> MASMETSSSCESLGSQPAAARPPSVDSLSSASTSHSENSVHTKSASVVSSDSISTSADNFSPDLRVLRESNKLAEMEEPPLLPGENIKDMAKDVTYICPFTGAVRGTLTVTNYRLYFKSMERDPPFVLDASLGVINRVEKIGGASSRGENSYGLETVCKDIRNLRFAHKPEGRTRRSIFENLMKYAFPVSNNLPLFAFEYKEVFPENGWKLYDPLLEYRRQGIPNESWRITKINERYELCDTYPALLVVPANIPDEELKRVASFR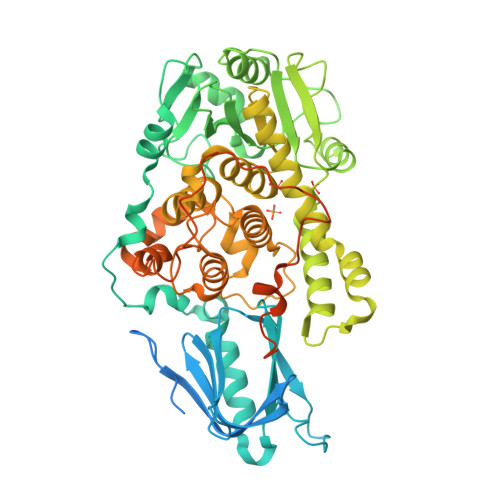SRGRIPVLSWIHPESQATITRCSQPMVGVSGKRSKEDEKYLQAIMDSNAQSHKIFIFDARPSVNAVANKAKGGGYESEDAYQNAELVFLDIHNIHVMRESLRKLKEIVYPNIEETHWLSNLESTHWLEHIKLILAGALRIADKVESGKTSVVVHSSDGWDRTAQLTSLAMLMLDGYYRTIRGFEVLVEKEWLSFGHRFQLRVGHGDKNHADADRSPVFLQFIDCVWQMTRQFPTAFEFNEYFLITILDHLYSCLFGTFLCNSEQQRGKENLPKRTVSLWSYINSQLEDFTNPLYGSYSNHVLYPVASMRHLELWVGYYIRWNPRMKPQEPIHNRYKELLAKRAELQKKVEELQREISNRSTSSSERASSPAQCVTPVQTVVAAALEHHHHHH> GMATDGLHENETLASLKSEAESLKGKLEEERAKLHDVELHQVAERVEALGQFVMKTRRTLKGHGNKVLCMDWCKDKRRIVSSSQDGKVIVWDSFTTNKEHAVTMPCTWVMACAYAPSGCAIACGGLDNKCSVYPLTFDKNENMAAKKKSVAMHTNYLSACSFTNSDMQILTASGDGTCALWDVESGQLLQSFHGHGADVLCLDLAPSETGNTFVSGGCDKKAMVWDMRSGQCVQAFETHESDVNSVRYYPSGDAFASGSDDATCRLYDLRADREVAIYSKESIIFGASSVDFSLSGRLLFAGYNDYTINVWDVLKGSRVSILF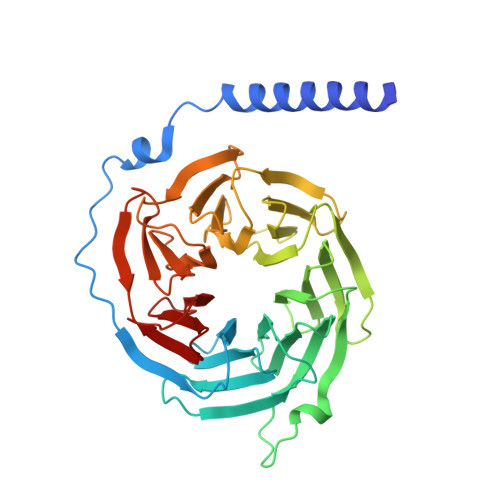GHENRVSTLRVSPDGTAFCSGSWDHTLRVWA> KSPSAQELKEQGNRLFVGRKYPEAAA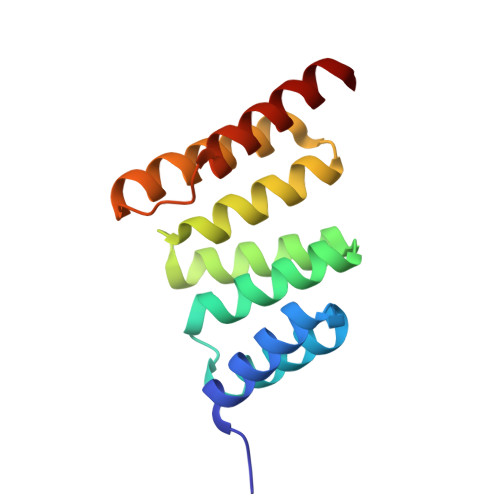CYGRAITRNPLVAVYYTNRALCYLKMQQHEQALADCRRALELDGQSVKAHFFLGQCQLEMESYDEAIANLQRAYSLAKEQRLNFGDDIPSALRIAKKKRWNS> GSGSMETLCQRLNVCQDKILTHYENDSTDLRDHIDYWKHMRLECAIYYKAREMGFKHINHQVVPTLAVSKNKALQAIELQLTLETIYNSQYSNEKWTLQDVSLEVYLTAPTGCIKKHGYTVEVQFDGDICNTMHYTNWTHIYICEEASVTVVEGQ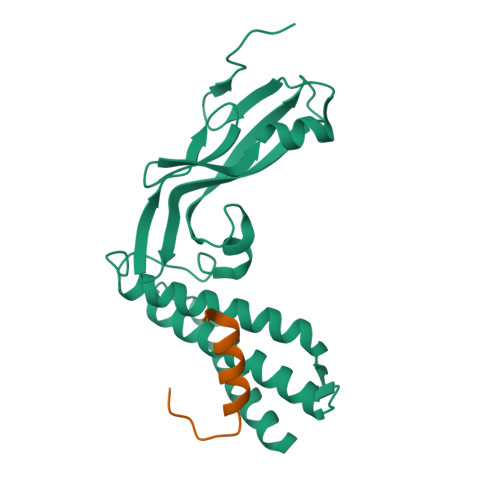VDYYGLYYVHEGIRTYFVQFKDDAEKYSKNKVWEVHAGGQVILCPTSVFS;> GSATIDMNFQSDLLSIFEENLF> MVFKKVLLTGTSEESFTAAADDAIDRAEDTLDNVVWAEVVDQGVEIGAVEERTYQTEVQVAFELDGSQLEHHHHHH

Dodecin from Halobacterium salinarum is a hollow spherical dodecameric protein, which binds oxidized flavins with high affinity, whereas flavin reduction induces the dissociation of the holoprotein. Herein we use the riboflavin binding protein dodecin as a redox-sensitive probe to study ET processes through DNA monolayers. To study ET, dodecin can be reconstituted on flavin-terminated ds-DNA adsorbed on gold electrodes. If ET through DNA is possible, applying a negative potential will result in flavin reduction and subsequent release of apododecin.

Prior to adsorption of apododecin tE, a non-binding dodecin variant dA was added as a negative control to show that apododecin tE is bound specifically to the flavins.5b To minimize the ET distance between the redox-active isoalloxazine subunit of flavin and DNA, different flavin–DNA ligands comprising only the first five bases at the 5′ end (oligo 5, O5) and flavins of different lengths (CofCn) were synthesized. Dodecin was reconstituted with these ligands and X-ray structures were measured. For all the flavin–DNA ligands, electron density can be traced for the isoalloxazine moiety (and the first two CH2 groups). For the CofC2_O5 ligand further electron density indicates binding between apoprotein and linker plus the first two DNA bases. As shown by superposition of the ligands in Figure 1 B, the (rather deep) position of the isoalloxazine ring of CofC2_O5 in the binding pocket is similar to that of lumiflavin, while all the other flavin–DNA hybrid ligands superimpose with riboflavin. Efficient ET could be observed even for larger distances between isoalloxazine and “molecular wires”, when the flavoenzyme glucose oxidase was reconstituted on gold electrodes, but using molecules other than DNA (e.g. single-walled carbon nanotubes) as the molecular wire.5f, 9 In the X-ray structures there was no electron density for most of the linker between DNA and flavin indicating that (also after protein reconstitution) different orientations of DNA and redox-center relative to each other are possible.>MQPDMSLNVIKMKSSDFLESAELDSGGFGKVSLAFHRTQGLMIMKTVYKGPNCIEHNEALLEEAKMMNRLRHSRVVKLLGVIIEEGKYSLVMEYMEKGNLMHVLKAEMSTPLSVKGRIILEIIEGMAYLHGKGVIHKDLKPENILVDNDFHIKIADLGLASFKMWSKLNNEEHNELREVDGTAKKNGGTLYYMAPEHLNDVNAKPTEKSDVYSFAVVLWAIFANKEPYENAIAEQQLIMAIKSGNRPDVDDITEYCPREIISLM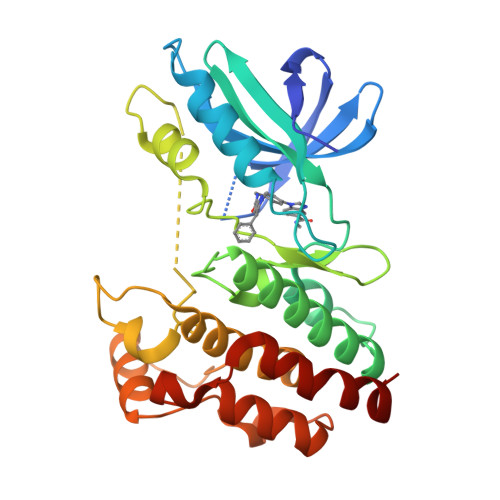KLCWEANPEARPTFPGIEEKFRPFYLSQLE[2x]>MKEKIIVSACLLGQPVRYDGQSKGIVSNWLDALGAEGRALAFCPEVAGGLPTPRPPAERQGEHVVTESGLDVTAEFDRGAELALGLCLAQGIRFALLKEGSPSCGSGRIYNGRFEGVSMAGEGKTTALLRRHGIQVFSEDQLPELALALSLVATAAGSLE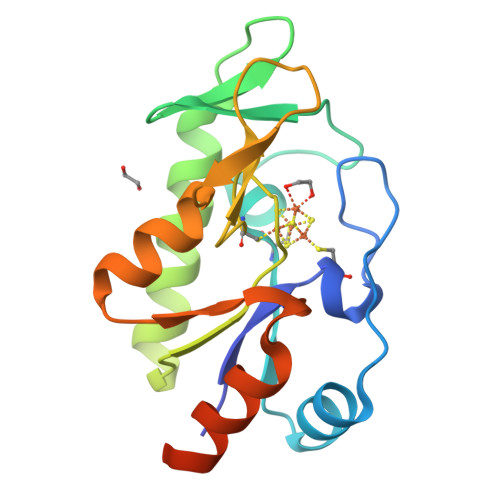HHHHHH[2x]>MNHKVHHHHHHMKANQVQPLNKYPVVFVHGFLGLVGDNAPALYPNYWGGNKFKVIEELRKQGYNVHQASVSAFGSNYDRAVQLYYYIKGGRVDYGAAHAAKYGHERYGKTYKGIMPNWEPGKKVHLVGHSMGGQTIRLMEEFLRNGNKEEIAYHQAHGGEISPLFTGGHNNMVASITTLATPHNGSQAADKFGNTEAVRKIMFALNRFMGNKYSNIDLGLTQWGFKQLPNESYIDYIKRVSKSKIWTSDDNAAYDLTLDGSAKLNNMTSMNPNITYTTYTGVSSHTGPLGYENPDLGTFFLMDTTSRIIGHDAREEWRKNDGVVPVISSLHPSNQPFVNVTNNEPATRRGIWQVKPILQGWDHVDFIGVDFL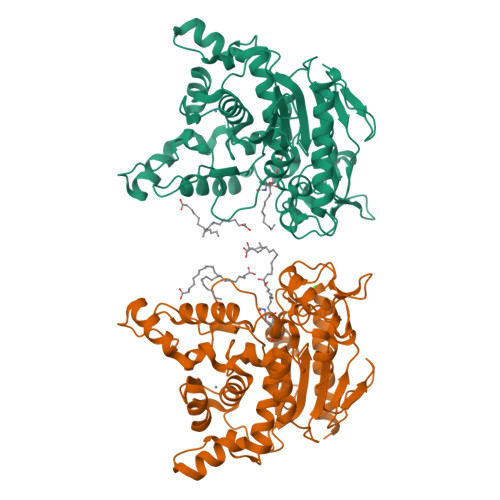DFKRKGSELANFYIGIINDLLSVEATEGKGTQLKAS[2x]>AAFKPEELRQALMPTLEALYRQDPESLPFRQPVDPQLLGIPDYFDIVKNPMDLSTIKRKLDTGQYQEPWQYVDDVWLMFNNAWLYNRKTSRVYKFC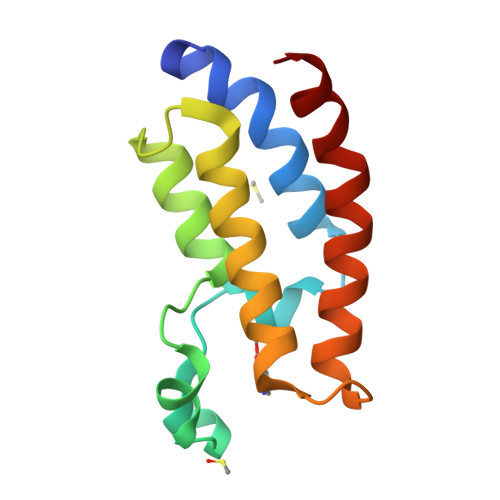SKLAEVFEQEIDPVMQSL[4x]> GSMGNLFGHKRWYEVRDKKDFKIKRKVKVKRNYDGNKYILNINENNNKEKIDNNKFIRKYINYKKNDNILKEFTRKFHAGNILFKLKGKEGIIRIENNDDFLETEEVVLYIEAYGKSEKLKALGITKKKIIDEAIRQGITKDDKKIEIKRQENEEEIEIDIRDEYTNKTLNDCSIILRIIENDELETKKSIYEIFKNINMSLYKIIEKIIENETEKVFENRYYEEHLREKLLKDDKIDVILTNFMEIREKIKSNLEILGFVKFYLNVGGDKKKSKNKKMLVEKILNINVDLTVEDIADFVIKELEFWNITKRIE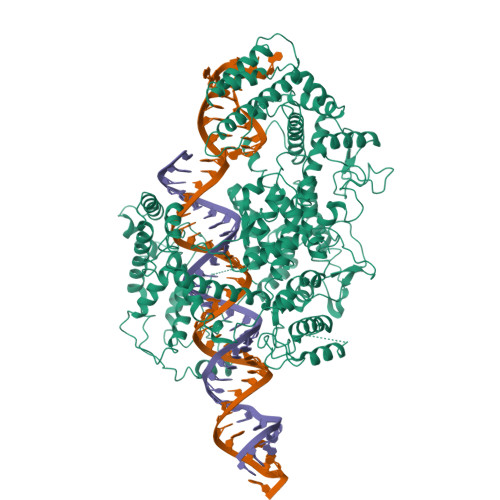KVKKVNNEFLEKRRNRTYIKSYVLLDKHEKFKIERENKKDKIVKFFVENIKNNSIKEKIEKILAEFKIDELIKKLEKELKKGNCDTEIFGIFKKHYKVNFDSKKFSKKSDEEKELYKIIYRYLKGRIEKILVNEQKVRLKKMEKIEIEKILNESILSEKILKRVKQYTLEHIMYLGKLRHNDIDMTTVNTDDFSRLHAKEELDLELITFFASTNMELNKIFSRENINNDENIDFFGGDREKNYVLDKKILNSKIKIIRDLDFIDNKNNITNNFIRKFTKIGTNERNRILHAISKERDLQGTQDDYNKVINIIQNLKISDEEVSKALNLDVVFKDKKNIITKINDIKISEENNNDIKYLPSFSKVLPEILNLYRNNPKNEPFDTIETEKIVLNALIYVNKELYKKLILEDDLEENESKNIFLQELKKTLGNIDEIDENIIENYYKNAQISASKGNNKAIKKYQKKVIECYIGYLRKNYEELFDFSDFKMNIQEIKKQIKDINDNKTYERITVKTSDKTIVINDDFEYIISIFALLNSNAVINKIRNRFFATSVWLNTSEYQNIIDILDEIMQLNTLRNECITENWNLNLEEFIQKMKEIEKDFDDFKIQTKKEIFNNYYEDIKNNILTEFKDDINGCDVLEKKLEKIVIFDDETKFEIDKKSNILQDEQRKLSNINKKDLKKKVDQYIKDKDQEIKSKILCRIIFNSDFLKKYKKEIDNLIEDMESENENKFQEIYYPKERKNELYIYKKNLFLNIGNPNFDKIYGLISNDIKMADAKFLFNIDGKNIRKNKISEIDAILKNLNDKLNGYSKEYKEKYIKKLKENDDFFAKNIQNKNYKSFEKDYNRVSEYKKIRDLVEFNYLNKIESYLIDINWKLAIQMARFERDMHYIVNGLRELGIIKLSGYNTGISRAYPKRNGSDGFYTTTAYYKFFDEESYKKFEKICYGFGIDLSENSEINKPENESIRNYISHFYIVRNPFADYSIAEQIDRVSNLLSYSTRYNNSTYASVFEVFKKDVNLDYDELKKKFKLIGNNDILERLMKPKKVSVLELESYNSDYIKNLIIELLTKIENTNDTL> GSGQSLNPHNDYCQHFVDTGHRPQNFIRDVGLADRFEEYPKLRELIRLKDELIAKSNTPPMYLQADIEAFDIRELTPKFDVILLEPPLEEYYRETGITANEKCWTWDDIMKLEIDEIAAPRSFIFLWCGSGEGLDLGRVCLRKWGYRRCEDICWIKTNKNNPGKTKTLDPKAVFQRTKEHCLMGIKGTVKCSTDGDFIHANVDIDLIITEEPEIGNIEKPVEIFHIIEHFCLGRRRLHLFGRDSTIRPGWLTVGPTLTNSNYNAETYASYFSAPNSYLTGCTEEIERLRPKSPPPKSKSDRGGGAPRGGGRGG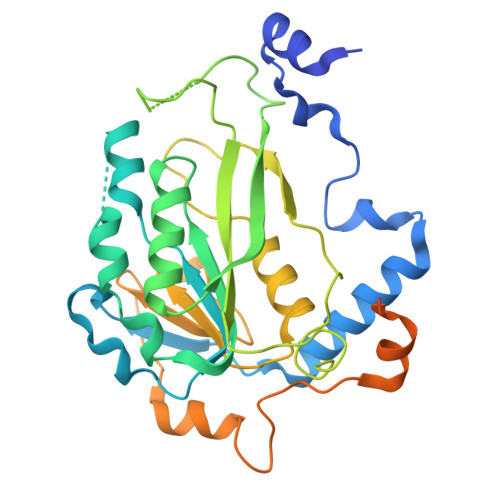TSAGRGRERNRSNFRGERGGFRGGRGGAHRGGFPPR Vesicular stomatitis virus (VSV) is a negative-strand RNA virus with a non-segmented genome, closely related to rabies virus. The VSV RNP complex assembles, together with M, into a helical, bullet-shaped structure, as it buds through the plasma membrane of an infected cell. The asymmetric unit of the VSV helical nucleocapsid, which repeats every 9 RNA nucleotides, contains one nucleoprotein (N) subunit and two (chemically identical) matrix protein subunits (M1 and M2). N is an elongated, two-lobed protein of ~420 amino-acid residues; the single stranded RNA binds in a cleft between the two lobes, with nine nucleotides per N subunit.

We obtained a helical reconstruction of the trunk at 4.1 Å resolution, and a local reconstruction of the basic building module (one N and two M proteins) at 3.5 Å resolution. We also calculated a local reconstruction by alignment and averaging of the asymmetric units (N subunit, 9 bound RNA nucleotides, and the two matrix protein subunits M1 and M2) from all N classes, yielding a nominal resolution of 3.5 Å. This map was then used to build and refine a molecular model of the asymmetric unit. We modeled the RNA nucleotides as poly-uridine, because the density in our reconstruction is the average of different sequences. Conserved residues NArg143, NLys206, NArg214, NLys286, NArg408, all ordered in our reconstruction with well-resolved side chain density, coordinate the phosphate groups of the RNA backbone by salt bridges. Conserved NTyr152 hydrogen-bonds to the phosphate group of nucleotide 8, and stacks with its aromatic side chain onto the sugar ring of nucleotide 6. Each N protein contacts three M1 subunits. The first of these radial inter-layer contacts, interface i, is the most extended, and the one that is also present in the tip of the VSV bullet (see below). The contact is well resolved in our local reconstruction and involves N protein residues 116–125 from a long loop that wraps around the N lobe domain and binds two M1 subunit loops, residues 94–101 and 149–152. Stabilizing interactions include hydrogen bonds between the main chain of the N loop 116–125 with the M1 loop 94–101. We also observe hydrophobic contacts between residues NVal121 and M1Met98 and NVal116-NLeu117-NPro118 and M1Pro149-M1Pro150.

>MSVTVKRIIDNTVIVPKLPANEDPVEYPADYFRKSKEIPLYINTTKSLSDLRGYVYQGLKSGNVSIIHVNSYLYGALKDIRGKLDKDWSSFGINIGKAGDTIGIFDLVSLKALDGVLPDGVSDASRTSADDKWLPLYLLGLYRVGRTQMPEYRKKLMDGLTNQCKMINEQFEPLVPEGRDIFDVWGNDSNYTKIVAAVDMFFHMFKKHECASFRYGTIVSRFKDCAALATFGHLCKITGMSTEDVTTWILNREVADEMVQMMLPGQEIDKADSYMPYLIDFGLSSKSPYSSVKNPAFHFWGQLTALLLRSTRARNARQPDDIEYTSLTTAGLLYAYAVGSSADLAQQFCVGDNKYTPDDSTGGLTTNAPPQGRDVVEWLGWFEDQNRKPTPDMMQYAKRAVMSLQGLREKTIGKYAKSEFDK[3x];>[3x]MSSLKKILGLKGKGKKSKKLGIAPPPYEEDTSMEYAPSAPIDKSYFGVDEMDTYDPNQLRYEKFFFTVKMTVRSNRPFRTYSDVAAAVSHWDHMYIGMAGKRPFYKILAFLGSSNLKATPAVLADQGQPEYHAHCEGRAYLPHRMGKTPPMLNVPEHFRRPFNIGLYKGTIELTMTIYDDESLEAAPMIWDHFNSSKFSDFREKALMFGLIVEKKASGAWVLDSISHFK> MADEATRRVVSEIPVLKTNAGPRDRELWVQRLKEEYQSLIRYVENNKNADNDWFRLESNKEGTRWFGKCWYIHDLLKYEFDIEFDIPITYPTTAPEIAVPELDGKTAKMYRGGKIKLTDHFK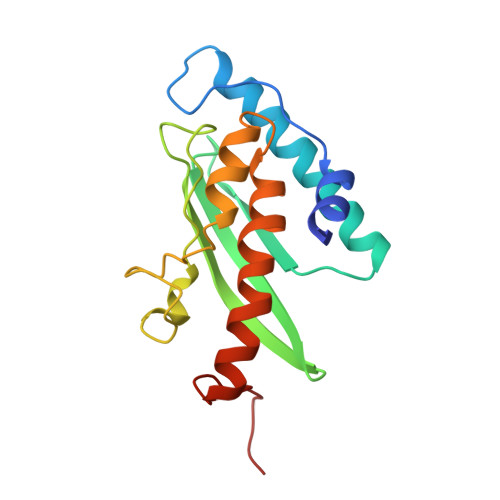PLWARNVPKFGLAHLMALGLGPWLAVEIPDLIQKGVIQHKEKCNQG(4R)-ISONICOTINIC-ACETYL-NICOTINAMIDE-ADENINE DINUCLEOTIDE | C27 H33 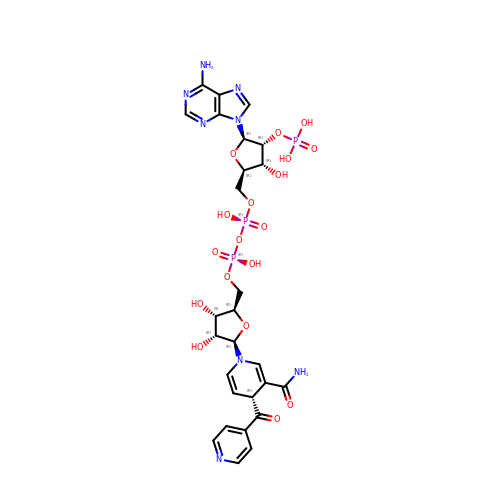N8 O18 P3 | FPZCWRGJBUDVSB-MXUAFQDZSA-N> SNAMSAGEVERLVSE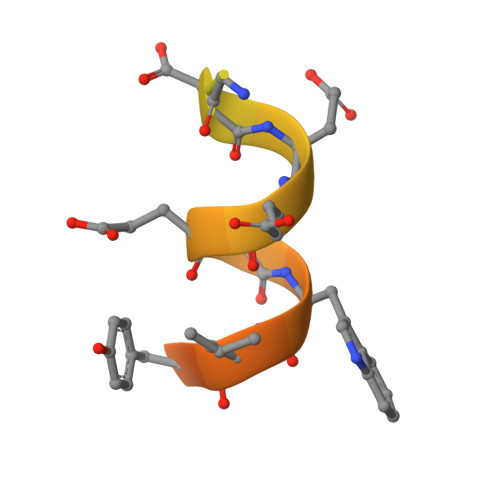LSGGTGGDEEEEWLYGDENEVER>WNGKGSTVDFQEIILRRCYTYIRVVQPELGDRDCQKIKKAFTDAFISKDPCSAREEDYDLLMKLGHQTVPCDKTVFWSKTKELAHQYTKTQKGLFTLENTLLGYIADDLSWCGKVGSSEINLESCPDRRNCNSNFVSVFWNLLSKRFAENACGMVQVFLNGSISNAFDKTSTFGRVEVHSLQPSKVHTLKAWVIHDSGKTPRDTCSGSSINELQLILRGKNIK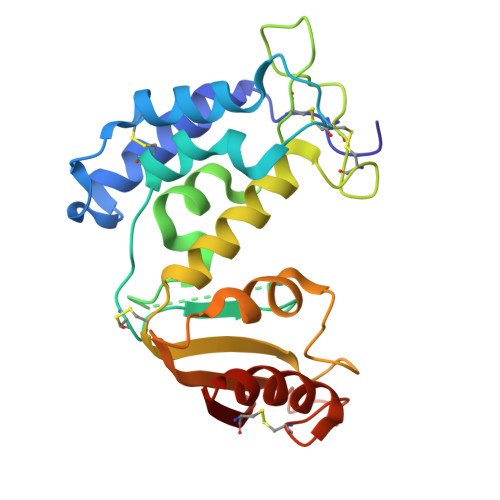FTCQENYRP[2x]2-(difluoromethoxy)-1-[(3aR,6aS)-hexahydrocyclopenta[c]pyrrol-2(1H)-yl]ethan-1-one 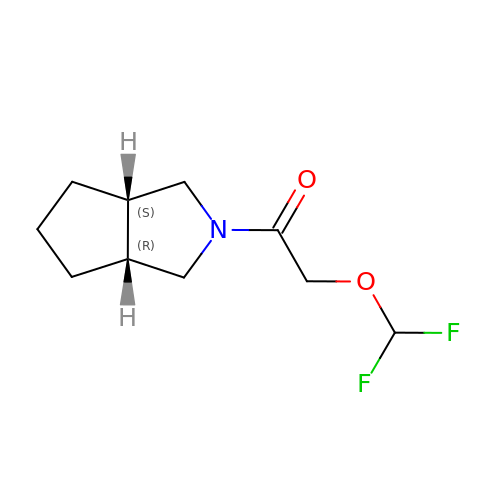| C10 H15 F2 N O2 | GFKMUMPBDKROCT-OCAPTIKFSA-N4-[(4,4-dimethylpiperidin-1-yl)methyl]-2-oxidanyl-~{N}-[[(3~{R})-3-oxidanyl-1-[6-[(phenylmethyl)amino]pyrimidin-4-yl]piperidin-3-yl]methyl]benzamide 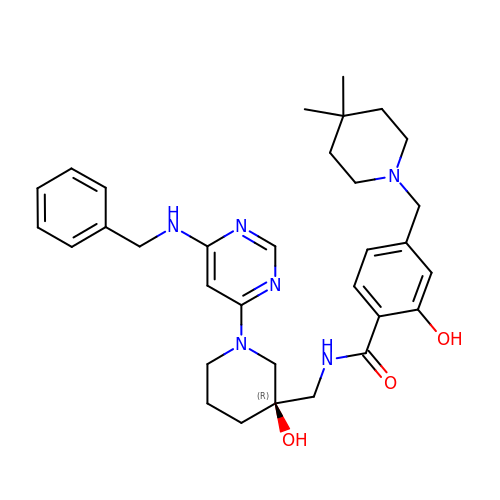| C32 H42 N6 O3 | PWYRDVXYAOGDNK-JGCGQSQUSA-N>SKEYHIDEEVGFALPNPQENLPDFYNDWMFIAKHLPDLIESGQLRERVEKLNMLSIDHLTDHKSQRLARLVLGCITMAYVWGKGHGDVRKVLPRNIAVPYCQLSKKLELPPILVYADCVLANWKKKDPNKPLTYENMDVLFSFRDGDCSKGFFLVSLLVEIAAASAIKVIPTVFKAMQMQERDTLLKALLEIASCLEKALQVFHQIHDHVNPKAFFSVLRIYLSGWKGNPQLSDGLVYEGFWEDPKEFAGGSAGQSSVFQCFDVLLGIQQTAGGGHAAQFLQDMRRYMPPAHRNFLCSLESNPSVREFVLSKGDAGLREAYDACVKALVSLRSYHLQIVTKYILIPASQQPKENKTSEDPSKLEAKGTGGTDLM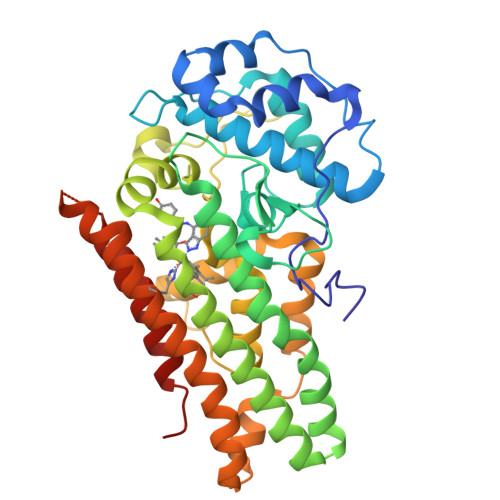NFLKTVRSTTEKSLLKEG[2x]>GSESSSQAVVVAIDAKRVDGEFMVFTYSGKKNTGILLRDWVVEVEKRGAGEILLTSIDRDGTKSGYDTEMIRFVRPLTTLPIIASGGAGKMEHFLEAFLRGADKVSINTAAVENPSLITQIAQTFGSQAVVVAIDAKRVDGEFMVFTYSGKKNTGILLRDWVVEVEKRGAGEILL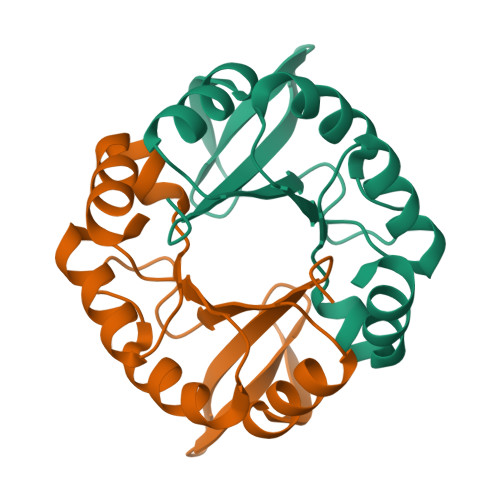TSIDRDGTKSGYDTEMIRFVRPLTTLPIIASGGAGKMEHFLEAFLRGADKVSINTAAVENPSLITQIAQTFG[2x]>MGNDRLHNGGFRLIISQELGHVTSRNNYQVVLDHSSVNFHTGAHIPLNELKDYIFGSSIRTIDYSASSDKIKVVKSANIVLFTRIFYLNEKSTLRIAISCCVTDDVLPVLTECWPHISSFLDQCENTLLKYLAKNDTQFLPHDWKARNCIEVA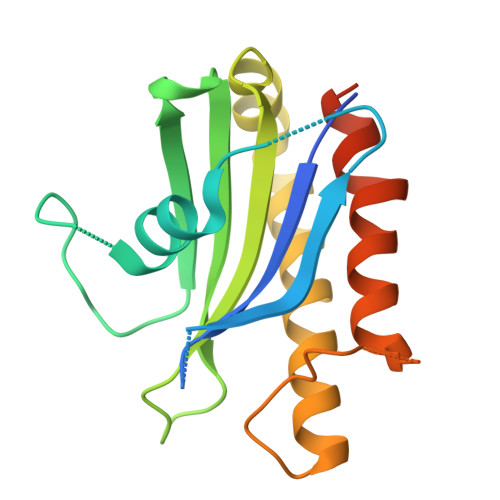AVLQTFQRKIIPLLSGYSLEGSHHHHHH[4x]> HEVVKFMDVYQRSYCHPIETLVDIFQEYPDEIEYIFKPSCVPLMRCGGCCNDEGLECVPTEE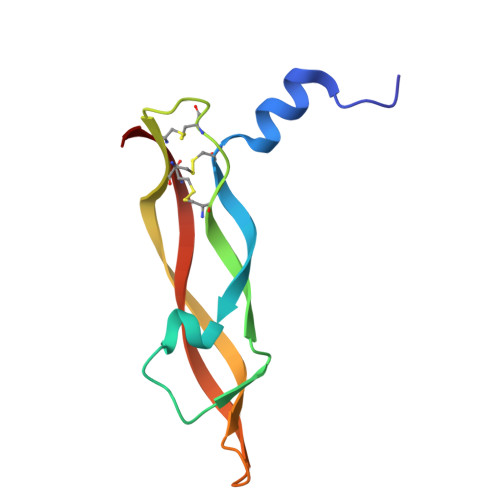SNITMQIMRIKPHQGQHIGEMSFLQHNKCECRPK> SGYSMTPPTLNITEESHVIDTGDSLSISCRGQHPLEWAWPGAQEAPATGDKDSEDTGVVRDCEGTDARPYCKVLLLHEVHANDTGSYVCYYKYIKARIEGTTAASSYVFVRDFEQPFINKPDTLLVNRKDAMWVPCLVSIPGL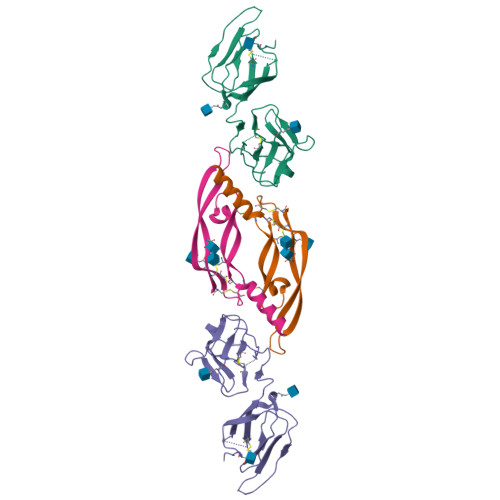NVTLRSQSSVLWPDGQEVVWDDRRGMLVSTPLLHDALYLQCETTWGDQDFLSNPFLVHITGNELADPIEGR;> DPTEETIKFAAAHYNTEILKSIDNEWRKTQCMPREVAIDVGKEFGVATNTFFKPPCVSVYRCGGCCNSEGLQCMNTSTSYLSKTLFEITVPLSQGPKPVTISFANHTSCRCMSKLHHHHHH4-[[(5~{S},7~{R})-3-azanyl-1-adamantyl]carbonylamino]-1~{H}-indole-2-carboxamide | C20 H24 N4 O2 | 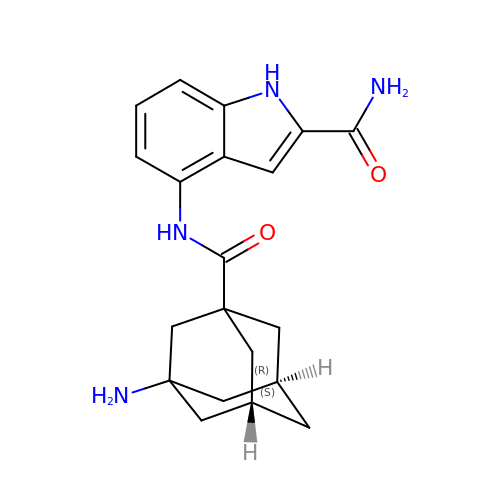WGKDLQGKGXBCBV-SRRICDNISA-N>[4x]GMSEPQRLFFAIDLPAEIREQIIHWRAKHFPPEAGRPVAADNLHLTLAFLGEVSA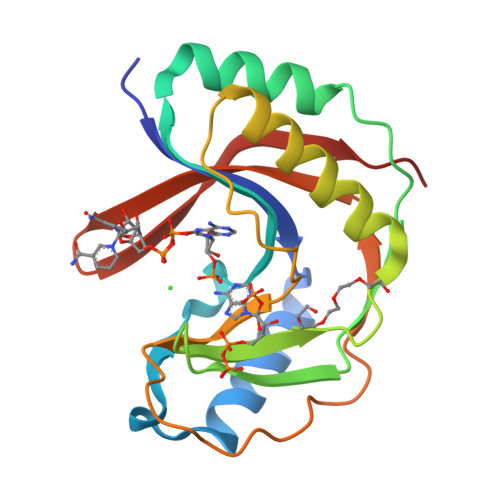EKEKALSLLAGRIRQPGFTLTLDDAGQWLRSRVVWLGMRQPPRGLIQLANMLRSQAARSGCFQSNRPFHPHITLLRDASEAVTIPPPGFNWSYAVTEFTLYASSFARGRTRYTPLKRWALTQ> MNQEEAIFRSADMTYVQLYIPLEVIREVTFLLGKMSVFMVMDLNKDLTAFQRGYVNQLRRFDEVERMVGFLNEVVEKHAAETWKYILHIDDEGNDIAQPDMADLINTMEPLSLENVNDMVKEITDCESRARQLDESLDSLRSKLNDLLEQRQVIFECSKFIEVNPGIAGRATNPEIEQEERDVDEFRMTPDDISETLSDAFSFDDETPQDRGALGNDLTRNQSVEDLSFLEQGYQHRYMITGSIRRTKVDILNRILWRLLRGNLIFQNFPIEEPLLEGKEKVEKDCFIIFTHGETLLKKVKRVIDSLNGKIVSLNTRSSELVDTLNRQIDDLQRILDTTEQTLHTELLVIHDQLPVWSAMTKREKYVYTTLNKFQQESQGLIAEGWVPSTELIHLQDSLKDYIETLGSEYSTVFNVILTNKLPPTYHRTNKFTQAFQSIVDAYGIATYKEINAGLATVVTFPFMFAIMFGDMGHGFILFLMALFLVLNERKFGAMHRDEIFDMAFTGRYVLLLMGAFSVYTGLLYNDIFSKSMTIFKSGWQWPSTFRKGESIEAKKTGVYPFGLDFAWHGTDNGLLFSNSYKMKLSILMGYAHMTYSFMFSYINYRAKNSKVDIIGNFIPGLVFMQSIFGYLSWAIVYKWSKDWIKDDKPAPGLLNMLINMFLAPGTIDDQLYSGQAKLQVVLLLA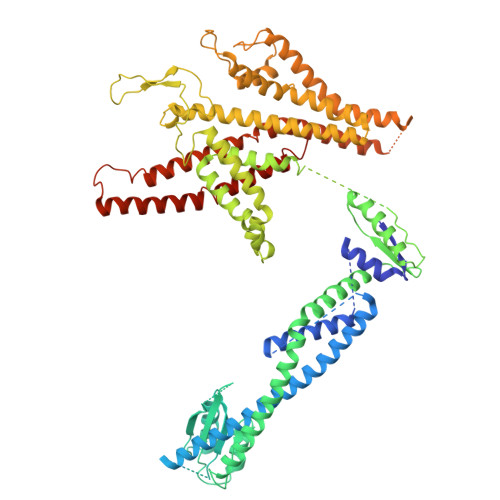ALVCVPWLLLYKPLTLRRLNKNGGGGRPHGYQSVGNIEHEEQIAQQRHSAEGFQGMIISDVASVADSINESVGGGEQGPFNFGDVMIHQVIHTIEFCLNCISHTASYLRLWALSLAHAQLSSVLWDMTISNAFSSKNSGSPLAVMKVVFLFAMWFVLTVCILVFMEGTSAMLHALRLHWVEAMSKFFEGEGYAYEPFSFRAIIE> GAAAD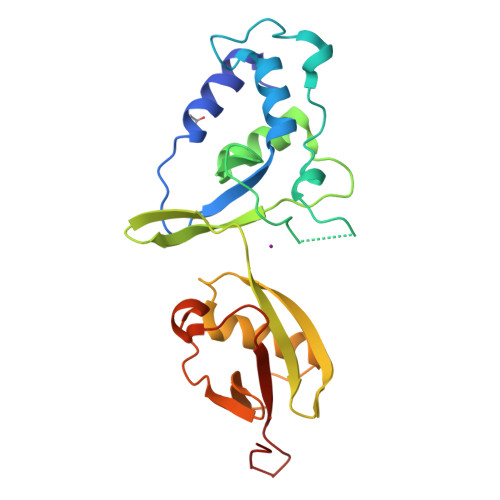LDTQRSDIATLLKTSLRKGDTWYLVDSRWFKQWKKYVGFDSWDKYQMGDQNVYPGPIDNSGLLKDGDAQSLKEHLIDELDYILLPTEGWNKLVSWYTLMEGQEPIARKVVEQGMFCKVEVYLTELKLCENGNMNNVVTRRFSKADTIDTIEKEIRKIFSIPDEKETRLWNKYMSNTFEPLNKPDSTIQDAGLYQGQVLVIEQKNEDGTWPRG(R)-(+) 5(9BH)-OXO-9B-PHENYL-2,3-DIHYDROTHIAZOLO[2,3-A]ISOINDOL-3-CARBOXYLIC ACID METHYL ESTER | C18 H15 N O3 S | 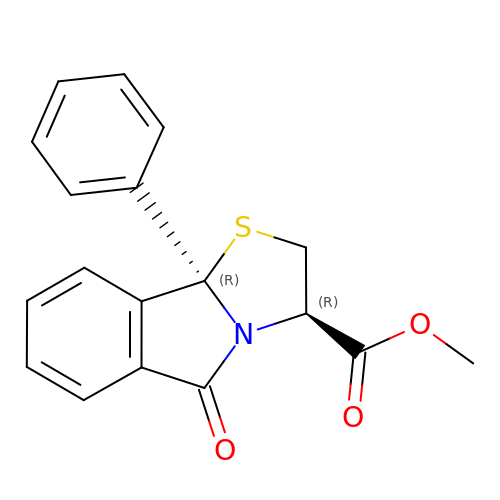JYIHODAXBBPFQF-MAUKXSAKSA-N>GMEEDIACVKDLVSKYLADNERLSRQKLAFLVQTEPRMLLMEGLKLLSLCIEIDSCNANGCEHNSEDKSVERILHDHGILTPSLCFVVPDGYKLTGNVLILLECFVRSSPANFEQKYIEDFKKLEQLKEDLKTVNISLIPLIDGRTSFYNEQIPDWVNDKLRDTLFSLLRY[2x]

Segmented negative strand RNA viruses of the arena-, bunya- and orthomyxovirus families uniquely carry out viral mRNA transcription by the cap-snatching mechanism. This involves cleavage of host mRNAs close to their capped 5′ end by an endonuclease (EN) domain located in the N-terminal region of the viral polymerase. The sNSV cap-snatching ENs belong to the PD-D/ExK superfamily of cation dependent nucleases. We find two different kinds of endonucleases, one with the characteristic catalytic histidine (His+) as in orthomyxovirus and bunyavirus, which have efficient endonuclease activity in isolation, and a second, without the histidine (His-) and conserved among arenaviruses which shows very poor activity in vitro.

To investigate the cause of the lack of activity of Lassa EN we structurally characterized the Mn2+ ion bound form by X-ray crystallography to see how it differs from the active ENs. Using a construct encompassing residues 1–174 from Lassa L protein we obtained three different crystal forms: one with no ions bound (crystal form X1), and two with one or two Mn2+ ions bound in the active site (crystal forms X2 and X3 respectively). Despite the presence of 2 mM MnCl2 in the crystallization buffer no anomalous scattering was detected in the active site. Compared with the X1 form, the X2 and X3 forms show a 17 degree rotation between the helical bundle lobe (residues 4–49 and 149–167) and residues 50–148, with the hinge being at the base of helix αb. The closure of the two lobes slightly changes the orientation of the active site residue E51. The previously reported Lassa EN structure in complex with Mg2+ ions has an open conformation of the two lobes, similar to the X1 apo-structure.>[2x]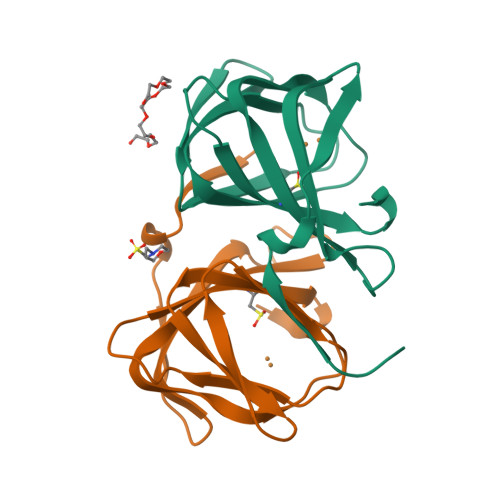GPSGMILKRAYDVTPQKISTDKVRGVRKRVLIGLKDAPNFVMRLFTVEPGGLIDRHSAPWEAEIFVLKGKLTVLKEQGEETVEEGFYIFVEPNEIHGFRNDTDSEVEFLCLIPKEGGE>[2x]QLPPSLPSDPRLWSREDVLVFLRFCVREFDLPKLDFDLFQMNGKRLCLLTRAD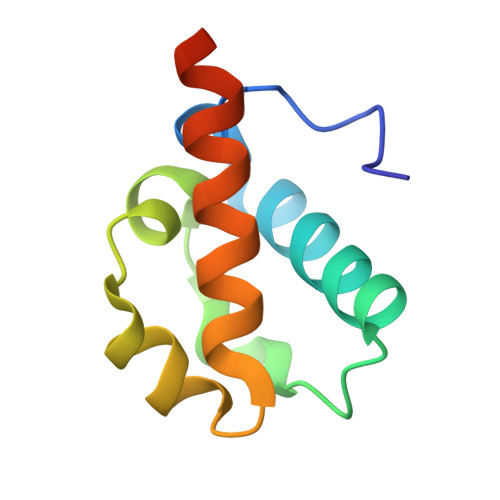FGHRCPGAGDVLHNVLQMLIIESHSRHHHHHH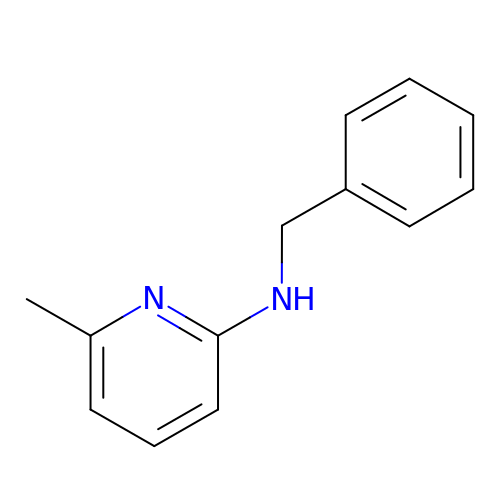6-methyl-~{N}-(phenylmethyl)pyridin-2-amine | C13 H14 N2 | FJZQUYGOKRVORO-UHFFFAOYSA-N>SQKSWIESTLTKRECVYIIPSSKDPHRCLPGCQICQQLVRCFCGRLVKQHACFTASLAMKYSDVKLGEHFNQAIEEWSVEKHTEQSPTDAYGVINFQGGSHSYRAKYVRLSYDTKPEIILQLLLKEWQMELPKLVISVHGGMQKFELHPRIKQLLGKGLIKAAVTTGAWILTGGVNTGVAKHVGDALKEHASRSSRKICTIGIAPWGVIENRNDLVGRDVVAPYQTLLNPLSKLNVLNNLHSHFILVDDGTVGKYGAEVRLRRELEKTINQQRIHARIGQGVPVVALIFEGGPNVILTVLEYLQESPPVPVVVCEGTGRAADLLAYIHKQTEEGGNLPDAAEPDIISTIKKTFNFGQSEAVHLFQTMMECMKKKELITVFHIGSEDHQDIDVAILTALLKGTNASAFDQLILTLAWDRVDIAKNHVFVYGQQWLVGSLEQAMLDALVMDRVSFVKLLIENGVSMHKFLTIPRLEELYNTKQGPTNPMLFHLIRDVKQGNLPPGYKITLIDIGLVIEYLMGGTYRCTYTRKRFRLIYNSLGGNNRRSGRNTSSSTPQLRKSHETFGNRADKKEKMRHNHFIKTAQPYRPKMDASMEEGKKKRTKDEIVDIDDPETKRFPYPLNELLIWACLMKRQVMARFLWQHGEESMAKALVACKIYRSMAYEAKQSDLVDDTSEELKQYSNDFGQLAVELLEQSFRQDETMAMKLLTYELKNWSNSTCLKLAVSSRLRPFVAHTCTQMLLSDMWMGRLNMRKNSWYKVILSILVPPAILMLEYKTKAEMSHIPQSQDAHQMTMEDSENNFHNITEEIPMEVFKEVKILDSSDGKNEMEIHIKSKKLPITRKFYAFYHAPIVKFWFNTLAYLGFLMLYTFVVLVKMEQLPSVQEWIVIAYIFTYAIEKVREVFMSEAGKISQKIKVWFSDYFNVSDTIAIISFFVGFGLRFGAKWNYINAYDNHVFVAGRLIYCLNIIFWYVRLLDFLAVNQQAGPYVMMIGKMVANMFYIVVIMALVLLSFGVPRKAILYPHEEPSWSLAKDIVFHPYWMIFGEVYAYEIDVCANDSTLPTICGPGTWLTPFLQAVYLFVQYIIMVNLLIAFFNQVYLQVKAISNIVWKYQRYHFIMAYHEKPVLPPPLIILSHIVSLFCCVCKRRKKDKTSDGPKLFLTEEDQKKLHDFEEQCVEMYFDEKDDKFNSGSEERIRVTFERVEQMSIQIKEVGDRVNYIKRSLQSLDSQIGHLQDLSALTVDTLKTLTAQKASEASKVHNEITRELSISKHLAQNLID[4x]

The transient receptor potential channel TRPM7 is a master regulator of the organismal balance of divalent cations that plays an essential role in embryonic development, immune responses, cell mobility, proliferation, and differentiation. TRPM7 represents a master regulator of the cellular balance of divalent cations and mediates uptake of Zn2+, Mg2+ and Ca2+, which is required for the normal prenatal development and healthy adulthood. The TRPM7 structure represents a tetramer assembled of four identical subunits, with the overall architecture reminiscent of other TRPM channels. Each TRPM7 subunit consists of an intracellular N-terminal domain (NTD, residues 1–789), transmembrane domain (TMD, 839–1146), and cytosolic C-terminal domain (CTD, 1157–1230).

To confirm that it is VER binding to the vanilloid-like site that causes inhibition of TRPM7-mediated currents, we tested the ability of VER to trigger the closure of the TRPM7-N1098Q channel, structurally characterized as the open channel in the absence of ligands. First, we conducted functional analysis and confirmed that TRPM7-N1098Q retained sensitivity to VER and NS, albeit the potency of both inhibitors was substantially reduced. Similar to the ligand-free apo condition, the purified TRPM7-N1098Q protein subjected to cryo-EM in the presence of 100 μM VER was represented by a single class of particles. This time, however, the corresponding cryo-EM reconstruction yielded a 2.99-Å resolution structure in the closed state, TRPM7-N1098QVER-Closed, where the pore appeared to have a nearly identical size to the pores of TRPM7Closed and TRPM7VER-closed. Importantly, we found VER in TRPM7-N1098QVER-closed bound to the same vanilloid-like sites as in TRPM7VER-closed, strongly supporting the idea that these are the sites that mediate TRPM7 inhibition by VER. Overall, functional characterization of the mutant TRPM7 channels verifies our VER- and NS-bound structures and supports the idea that the vanilloid-like site serves as the primary inhibitory site in TRPM7.> SAGAGSHCQKTSLRVNFEDIGWDSWIIAPKEYEAYECKGGCFFPLADDVTPTKHAIVQTLVHLKFPTKVGKACCVPTKLSPISVLYKDDMGVPTLKYHYEGMSVAEC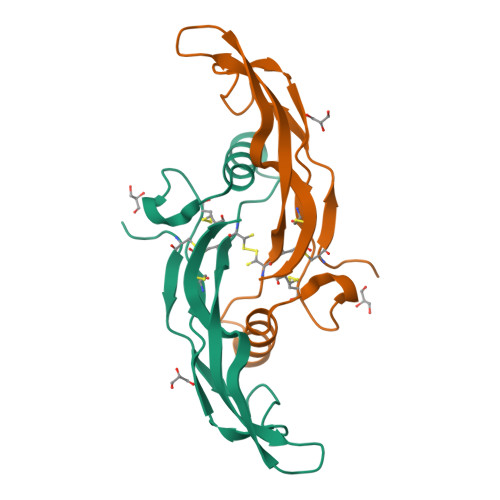GCR> QSESYKDAYSRINAIVIEGEQEAFDNYNRLAEMLPDQRDELHKLAKMEQRHMKGFMACGKNLSV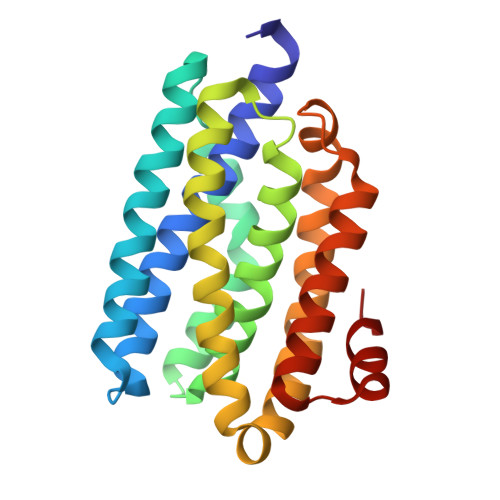TPDMGFAQKFFERLHENFKAAAAEGKVVTCLLIQSLIIECFAIAAFNIYIPVADAFARKITEGVVRDEYLHRNFGEEWLKANFDASKAELEEANRQNLPLVWLMLNEVADDARELGMERESLVEDFMIAYGEALENIGFTTREIMRMSAYG>[2x]MKYKEPFGVKLDFETGIIENAKKSVRRLSDMKGYFIDEEAWKKMVEEGDPVVYEVYAIEQEEKEGDLNFATTVLYPGKVGNEFFMTKGHYHS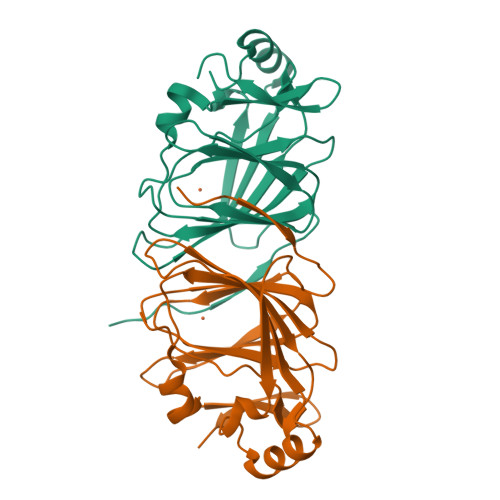KIDRAEVYFALKGKGGMLLQTPEGEARFIEMEPGTIVYVPPYWAHRTINTGDKPFIFLALYPADAGHDYGTIAEKGFSKIVVEENGKVVVKDNPKWRM>[2x]KNEETEKKLNLNQQRLGTVVAVLKSVNAKKVIDLGCGEGNLLSLLLKDKSFEQITGVDVSYSVLERAKDR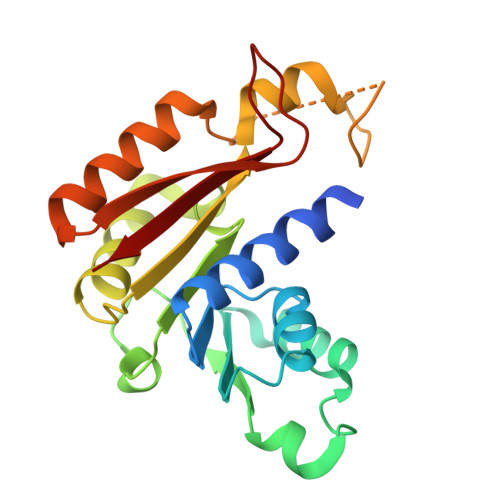LKIDRLPEMQRKRISLFQSSLVYRDKRFSGYDAATVIEVIEHLDENRLQAFEKVLFEFTRPQTVIVSTPNKEYNFHYQNLFEGNLRHRDHRFEWTRKEFETWAVKVAEKYGYSVRFLQIGEIDDEFGSPTQMGVFTL> MRGSHHHHHHGSQGLEGEDLEHLEQALKEVFGKGFKDLTPSDAVKLNMPAIAESGANVPAEVEVALPKEQVRAIHLFADKNPTPHILAFMPMKAEPYYATRVRLAETTAIRAVVETQ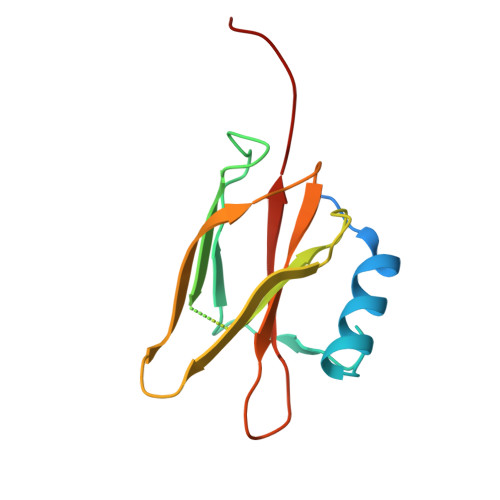DGKLLLASASTRVTVGGCG>MALIVQKFGGTSVGTVERIEQVAEKVKKFREA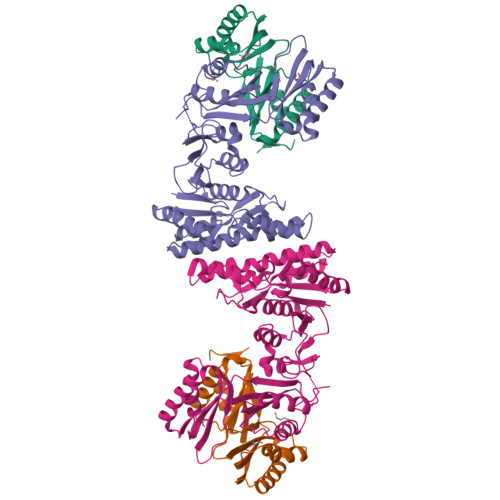GDDVVVVVSAMSGETNRLIGLANQIMEQPVPRELDVMVSTGEQVTIALLSMALIKRGVPAVSYTGNQVRILTDSAHTKARILHIDDTHIRADLKAGRVVVVAGFQGVDGNGNITTLGRGGSDTTGVALAAALKADECQIYTDVDGVYTTDPRVVPQARRLDKITFEEMLEMASLGSKVLQIRAVEFAGKYNVPLRVLHSFQEGPGTLITIDDEEESMEQPIISGIAFNRDEAKLTIRGVPDTPGVAFKILGPISAANVEVDMIVQNVAHDNTTDFTFTVHRNDYLNALEILKQTAANIGAREAIGDTNIAKVSIVGVGMRSHAGVASRMFEALAKESINIQMISTSEIKVSVVIEEKYLELAVRALHTAFELDAPARQGE[4x];>[4x]MEQPIISGIAFNRDEAKLTIRGVPDTPGVAFKILGPISAANVEVDMIVQNVAHDNTTDFTFTVHRNDYLNALEILKQTAANIGAREAIGDTNIAKVSIVGVGMRSHAGVASRMFEALAKESINIQMISTSEIKVSVVIEEKYLELAVRALHTAFELDAPARQGE>[3x]YSQTKADVVWKDVDGVSMPIPPKTHPRLYLREQQVPDLKNRMNDPKLKKVWADMIKMQEDWKPADIPEVKDFRFYFNQKGLTVRVELMALNYLMTKDPKVGREAITSIIDTLETATFKPAGDISRGIGLFMVTGAIVYDWCYDQLKPEEKTRFVKAFVRLAKMLECGYPPVKDKSIVGHASEWMIMRDLLSVGIAIYDEFPEMYNLAAGRFFKEHLVARNWFYPSHNYHQGMSYLNVRFTNDLFALWILD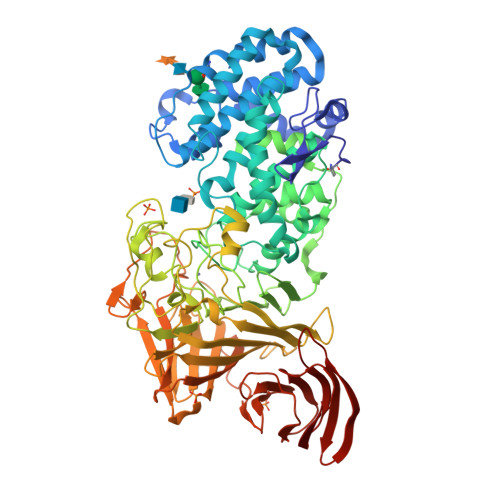RMGAGNVFNPGQQFILYDAIYKRRPDGQILAGGDVDYSRKKPKYYTMPALLAGSYYKDEYLNYEFLKDPNVEPHCKLFEFLWRDTQLGSRKPDDLPLSRYSGSPFGWMIARTGWGPESVIAEMKVNEYSFLNHQHQDAGAFQIYYKGPLAIDAGSYTGSSGGYNSPHNKNFFKRTIAHNSLLIYDPKETFSSSGYGGSDHTDFAANDGGQRLPGKGWIAPRDLKEMLAGDFRTGKILAQGFGPDNQTPDYTYLKGDITAAYSAKVKEVKRSFLFLNLKDAKVPAAMIVFDKVVASNPDFKKFWLLHSIEQPEIKGNQITIKRTKNGDSGMLVNTALLPDAANSNITSIGGKGKDFWVFGTNYTNDPKPGTDEALERGEWRVEITPKKAAAEDYYLNVIQIADNTQQKLHEVKRIDGDKVVGVQLADRIVTFSKTSETVDRPFGFSVVGKGTFKFVMTDLLPGTWQVLKDGKILYPALSAKGDDGALYFEGTEGTYRFLR>[4x]MRGSHHHHHTTGEDDESECVINYVEKAVNKLTLQMPYQLFIGGEFVDAEGSKTYNTINPTDGSVICQVSLAQVSDVDKAVAAAKEAFENGLWGKINARDRGRLLYRLADVMEQHQEELATIEALDAGAVYTLALKTHVGMSIQTFRYFAGWCDKIQGATIPINQARPNRNLTLTKKEPVGVCGIVIPWNYPLMMLSWKTAACLAAGNTVVIKPAQVTPLTALKFAELTLKAGIPKGVVNILPGSGSLVGQRLSDHPDVRKIGFTGSTEVGKHIMKSCALSNVKKVSLELGGKSPLIIFADCDLNKAVQMGMSSVFFNKGENCIAAGRLFVEESIHNQFVQKVVEEVEKMKIGNPLERDTNHGPQNHEAHLRKLVEYCQRGVKEGATLVCGGNQVPRPGFFFQPTVFTDVED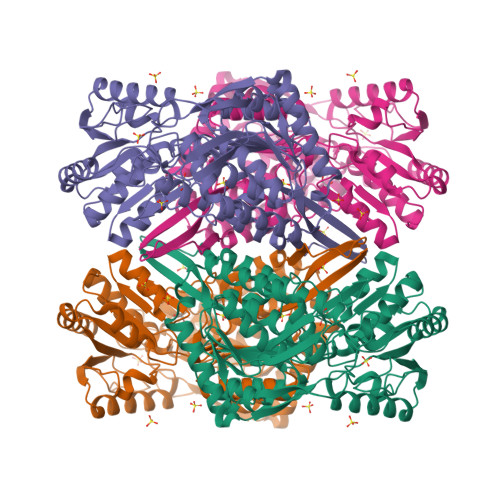HMYIAKEESFGPIMIISRFADGDVDAVLSRANATEFGLASGVFTRDINKALYVSDKLQAGTVFINTYNKTDVAAPFGGFKQSGFGKDLGEAALNEYLRIKTVTFEY(1E)-1-[5-TERT-BUTYL-2-(3-FLUOROPHENYL)-1H-PYRAZOL-3-YLIDENE]-3-(4-PYRIDIN-3-YLOXYPHENYL)UREA 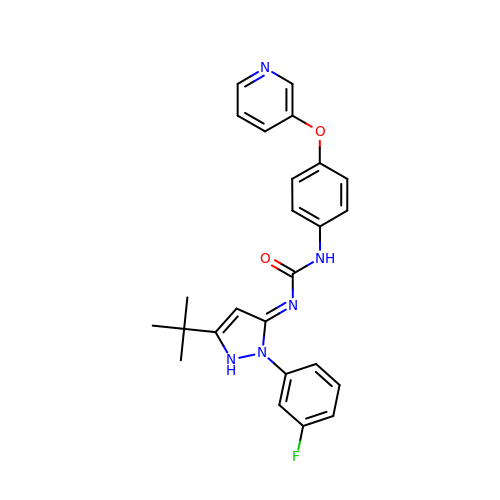| C25 H24 F N5 O2 | VWGLIDHWYMNSEW-BYNJWEBRSA-N>[2x]MNDIVSAKVLEYKGKKLNFTPEDPAEETIPADELHEHLQKPSTARTKRLKERCRWKHASAGEFIEKSVTAGIERMRYLTEAHKASEGKPEAIRRALGLANVLNKSTLVLQEDEFIVGYHAEDPNMFPLYPELSHMAVQDYLRSDYSPQPADEAAAINEYWKPHSLQSKCQPYFDPADLGRMYQVSSMEAPSFASGYNSIVPPYETVLEDGLLARIKLAEKHIAEAQADMSTFPWNGTKGLDNIAKIDNWKAMVIACKAVISWARRQGRLCKIVAENFETDPKRQAELLEIADICQRIPAEPCKGLKDAMQAKFFTFLICHAIERYASGYAQKEDTLLWPYYKASVVDKKFQPMSHMDAVELVEMERLKISEHGAGKSRAYREIFPGSNDLFILTVGGTNAKGEDACNDMTDAILEAAKRIRTAEPSIVFRYSKKNREKTLRWVFECIRDGLGYPSIKHDEIGTEQMKEYAKFSLNGNGATDEEAHNWVNVLCMSPGIHGRRKTQKTRSEGGGSIFPAKLLEISLNDGYDWSYADMQLGPKTGDLSSLKSFEDVWEAFRKQYQYAINLCISTKDVSRYFEQRFLQMPFVSAIDDGCMELGMDACALSEQPNGWHNPITTIVAANSLVAIKKLVFEEKKYTLEQLSQALKANWEGFEEMRVDFKRAPKWGNDDDYADGIITRFYEEIIGGEMRKITNYSGGPVMPTGQAVGLYMEVGSRTGPTPDGRFGGEAADDGGISPYMGTDKKGPTAVLRSVSKVQKNQKGNLLNQRLSVPIMRSKHGFEIWNSYIKTWHDLNIDHVQFNVVSTDEMRAAQREPEKHHDLIVRVSGYSARFVDIPTYGQNTIIARQEQDFSASDLEFLNVEISGTGSGSSHHHHHH;>MEGSNMETGQNLQNQPHTEVGTARPCRSCKWQTPDPTDPHRGQCTANRHAMGGVWKRWLRDVENTTCSRHEEGKLSFRDHV[2x];>MGTTTCKQCANFFPVPKDADDYEAGKADCVREKEDEKGKYWLSKPIFEN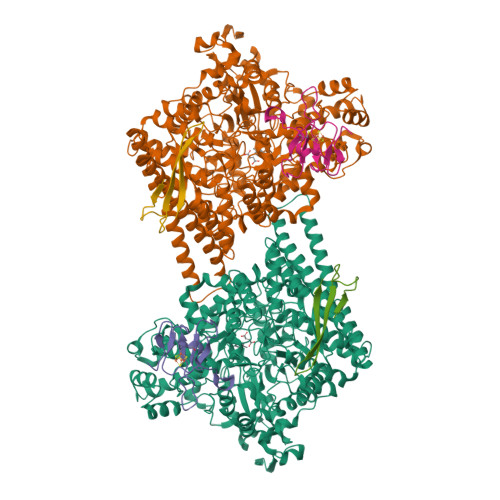SAQCEAFQTKR[2x]HYGROMYCIN B VARIANT | C20 H37 N3 O13 | 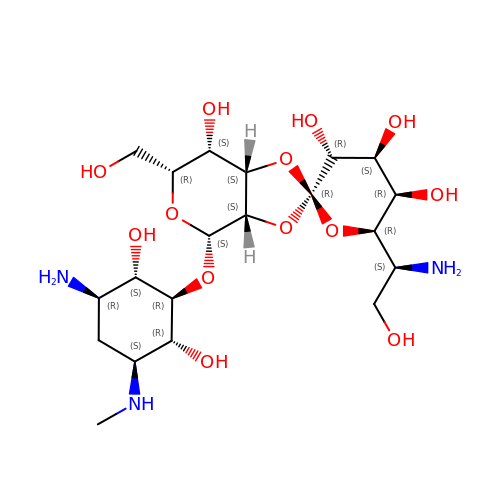GRRNUXAQVGOGFE-XFOBNZBXSA-N>[4x]SNIDHSKNNIIEEFDKLSDDFSNDINATKQTIKDLFLDIEASFEDTSDDVVKLLSKYSFVPEEKLNIIDGILRSFIENNKTHVINSSNAYIYIQKEKIKNVCNFILKKLNSLIQINELNKSHIILKYGKGEAKKGVLESIKNNDDISKNLKSELLKYENVNNQNIRVSELINFITPIYDDFIKNLTDLINDLQIKLKNISK

Two proteins from P. berghei, a rodent-infecting parasite, have been identified to be essential for host cell traversal by sporozoites. These are PbSPECT1 and PbSPECT2 (sporozoite microneme protein essential for cell traversal). No pore formation or host cell membrane wounding is seen in the absence of either of these proteins. In contrast to PbSPECT2, PbSPECT1 (∼25 kDa) has no detectable primary sequence homology to proteins of known structure or function.

A construct encoding PbSPECT1 residues 42–241, called PbSPECT1Δ41, was then expressed in E. coli and purified. Crystals of PbSPECT1Δ41 diffracted to 2.7 Å resolution, and its structure was determined by a combination of isomorphous replacement and multi-wavelength anomalous dispersion. The structure of PbSPECT1Δ41 revealed that it forms a four α-helix bundle with a ‘hook’-like feature at one end. In contrast to this pattern, the helices in PbSPECT1Δ41 are nearly parallel or antiparallel to one another; the angles between the helices range between 1–8° from parallel/antiparallel. Two PbSPECT1Δ41 molecules came together in a “V”-shaped arrangement, with a total of ∼1260 Å2 being buried at the interface. The asymmetric unit is constituted by two of these “V”-shaped, presumptive dimers that are then related by noncrystallographic translational symmetry. The segment leading from the “hook” to the α4 helix appears also to be flexible, as electron density for this region (residues 198–205) was visible in only one of the four PbSPECT1Δ41 molecules in the asymmetric unit; this electron density was sufficient for modeling only the main chain. In contrast, a striking and spacious cavity occurs in the interior of the structure proximal to the “hook”. The volume of this cavity is ∼750 Å3, but in actuality may be just somewhat smaller as six residues in the α1-α2 loop, which is at the top of the cavity, were not modeled. This cavity is lined predominantly by hydrophobic residues (L75, F76, I79, A81, S82, D89, V90, V91, L94, Y97, N156, K160, I163, I164, Y167, G168, K169, V207, L210, I214, I217, Y218, F221), with most of these being conserved in PbSPECT1 homologs. Of further note, this cavity is juxtaposed against an unusually deep pocket (145 Å2 in area) on the surface of PbSPECT1Δ41.>MQQLNENKIIKLLRDNIPKLQLIYLFGSYSQGTQHRNSEIEIAVLAADTLDNIARWELAQKLASALDSDVDLVDLRSASTVLCQQVVTQGKQLWGTQQDDELFAVKTISMYQHLQAERQAIIDDVMANTAAKAHRGESL[2x];>[6x]MNDIIINKIATIKRCIKRIQQVYGDGSQFKQDFTLQDSVILNLQRCCEACIDIANHINRQQQLGIPQSSRDSFTLLAQNNLITQPLSDNLKKMVGLRNIAVHDYQELNLDIVV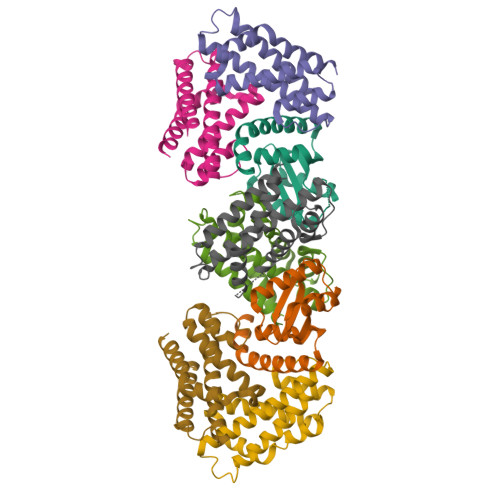HVVQHHLEDFEQFIDVIKAE>[2x]ETGSAQQLNEDLRLHLLLNTSVTCNDGSPAGYYLKESRGSRRWLLFLEGGWYCFNRENCDSRYDTMRRLMSSRDWPRTRTGTGILSSQPEENPYWWNANMVFIPYCSSDVWSGASSKSEKNEYAFMGALIIQEVVRELLGRGLSGAKVLLLAGSSAGGTGVLLNVDRVAE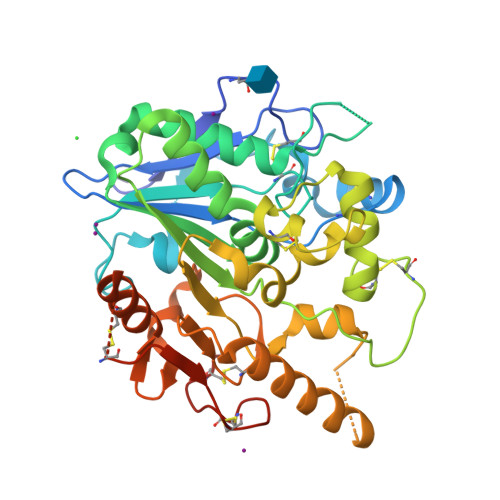QLEKLGYPAIQVRGLADSGWFLDNKQYRHTDCVDTITCAPTEAIRRGIRYWNGVVPERCRRQFQEGEEWNCFFGYKVYPTLRSPVFVVQWLFDEAQLTVDNVHLTGQPVQEGLRLYIQNLGRELRHTLKDVPASFAPACLSHEIIIRSHWTDVQVKGTSLPRALHCWDRSLHDSHKASKTPLKGCPVHLVDSCPWPHCNPSCPTGTKHHHHHH> GGHMTQVSKVATDARLTAQAQRLLVVSDNQELSLYLKEELEKQSFERPFNADFCYTSFNTNPQQMMAMGATKINIKDEFTVERIINEYDLVFSLHCKQIFPAKLTDNVCCINFHPGLNPYNRGWYPQAFSIINGLP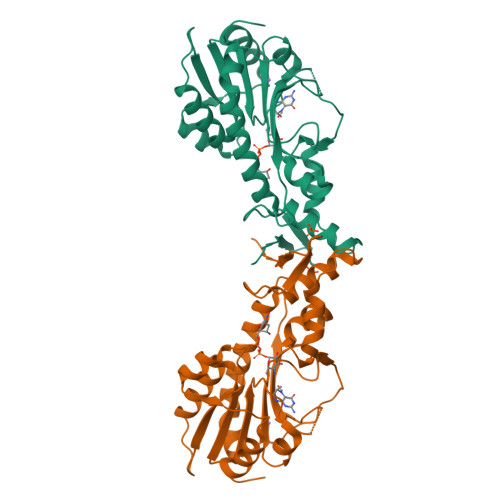TGATIHLMDAEVDHGDIIDQQEVEVKMSDTSLTVYRKVIAIEKHLISRNIFTIITRSYTTKKPQAEGNYNGIKDFNALCELDLNSIGTLDEHLKILRATTHGDFKNAFFCDEKGRRFFVRIVIDEAF>GPAGAQDDVPPYFKTEPVRTQVHLEGNRLVLTCMAEGSWPLEFKWLHNNRELTRFSLEYRYMITSLDRTHAGFYRCIVRNRMGALLQRQTEVQVAYMGSFEEGEKRQSVNHGEAAVIRAPRISSFPRPQVTWFRDGRKIPPSSRIAITLENTLVILSTVAPDAGRYYVQAVNDKNGDNKTSQPITLAVENVGGPADPIAPTIIIPPKNTSVVAGTSEVTMECVANARPLIKLHIVWKKDGAPLSSGISDYNRRLTIANPTVSDAGYYECEAMLRSSSVAPVTRGAYLSVLEPPQFVREPERHITAEMEKVVDIPCRAKGVPPPSITWYKDAALVEVGKLTRFKQRSDGGLQISGLLPDDTGMLQCFAHNAAGEAQTSTYLAVTS[2x]

Sdk1 and Sdk2 are single-pass transmembrane proteins, with extracellular regions composed of 6 N-terminal immunoglobulin (Ig) domains followed by 13 fibronectin type III (FNIII) domains, and a relatively short intracellular domain terminating in a Postsynaptic density/Discs Large/ZO-1 (PDZ) binding motif. Here, we report the crystal structures of cell-cell adhesive homophilic dimers of mouse Sdk1 and Sdk2, each mediated by the four N-terminal Ig domains. These four domains adopt a horseshoe conformation, like many other IgSF cell-cell recognition proteins, but they interact in a unique back-to-back anti-parallel manner not previously observed. Overall, our data suggest a model in which Sdks form cis dimers on isolated cell surfaces, which dissociate to form trans dimers through the same interface when contact is made to a cell surface expressing the cognate Sdk.

Two crystal forms of Sdk1Ig1–4 were determined at 2.2 and 3.2 Å resolution respectively, one of Sdk1Ig1–5 at 3.5 Å, two of Sdk2Ig1–4 at 2.7 and 3.2 Å respectively, and one of the Sdk2Ig1–2/Sdk1Ig3–4 chimera at 2.7 Å resolution. Although the Ig1–2:Ig1–2 interaction is present in all of the crystal forms of Sdk1 and Sdk2, there is a difference in rotational angle between the two horseshoes of the dimer among the crystal forms, with the Ig1–2:Ig1–2 interface acting as the hinge. The Ig3–4:Ig3–4 interaction varies from the Ig3–4 domains forming a considerable additional interface—as in Sdk1Ig1–4 crystal form 2 (915 Å2 BSA) and Sdk2Ig1–4 crystal form 1 (1294 Å2 BSA)—to being splayed 14 Å apart, as in the Sdk1Ig1–4 crystal form 1 structure (0 Å2 BSA). Analysis of the Ig3–4:Ig3–4 interface regions in the Sdk1Ig1–4 crystal form 2 and Sdk2Ig1–4 crystal form 1 structures, which show the most extensive Ig3–4:Ig3–4 contacts, reveals predominantly hydrophilic surfaces with hydrogen bonds between N253Ig3 and P287Ig4 in both structures, S240 Ig3 and T291Ig4 in Sdk1, and T255Ig3 and E286Ig4 in Sdk2. However, there are three Ig3–4:Ig3–4 interfacial residues that show non-conservative differences between Sdk1 and Sdk2 that are mostly conserved amongst vertebrate orthologs (H/S243Ig3, Y/Q289Ig4 and S/R296Ig4). These differences result in the Sdk2 interface containing a π-stacking interaction between Y245Ig3 and R296Ig4, which is absent from Sdk1. Mutagenesis of a key Ig3–4:Ig3–4 interface residue (N253E) did not prevent Sdk dimerization, although it did reduce the dimer affinity, particularly for Sdk2, which went from 2.2 μM to 18.9 μM, implying a small Ig3–4 contribution to dimer strength of around 1.3 kcal/mol. In addition to these major interfacial regions, the Sdk1Ig1–4 crystal form 2 also shows a small contact region between Ig1 residues E11 and R83 and Ig3 residue E212 towards the center of the horseshoe dimer. This interaction is not seen in either of the Sdk2 structures, although the residues are conserved.> MAHHHHHHMDCSTGAAIGQQFAKDAFHMHGGVGVGPTGNSEHDVLMNEMMMVQTPTGPAGEWTHQFAAYQGQQQQQQQQHPQELAMRHQQNDAFMLRQQQEMEEAFCTFCTTHPHSHAHSHQPQGLVGPAMMGPQIMPPMMFGPGTGGFMMGAPPMMPYASMKFAGDAAMAAANNTNMTQGATATSTTSVQQELQQQSSDNGWVEKLRDAEWAQDYSDAQVFTLEGQSEQTMEEHAKNSEFYQFMDKIRSKELLIDEETGQLVQGPGPDPDAPEDAEYLKEWAAAEGLNMPPGFFEHMMQRPQGNNEQAEGRLFDGSNDALMDDGALDNAADVEEWVREYA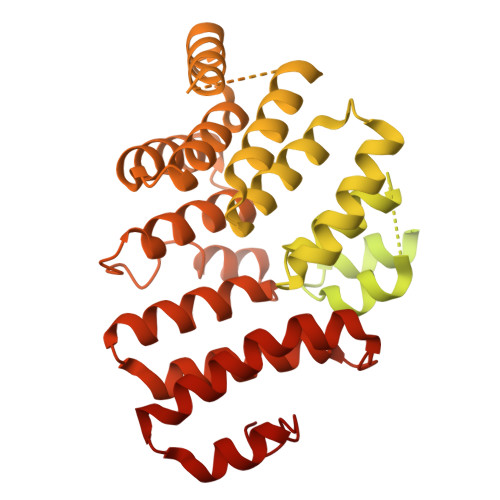EAQEQLQRVQNETNYPFEPNNPYMYHDKPMEEGIAMLQLANMAEAALAFEAVCQKEPENVEAWRRLGTTQAENEKDCLAIIALNHARMLDPKDIAVHAALAVSHTNEHNVGAALQSLRSWLLSQPQYEHLGLVDLREVAADEGLDEVPEENYFFAAPSEYRDCCTLLYAAVEMNPNDPQLHASLGVLHNLSHRFDEAAKNFRRAVELRPDDAHMWNKLGATLANGNRPQEALEAYNRALDINPGYVRVMYNMAVSYSNMAQYPLAAKHITRAIALQAGGTNPQGEGSRIATRGLWDLLRMTLNLMDRSDLVEASWQQDLTPFLREFGLEEMAV>[4x]SPFHLNDAVAIVTGAAAGIGRAIAGTFAKAGASVVVTDLKSEGAEAVAAAIRQAGGKAIGLECNVTDEQHREAVIKAALD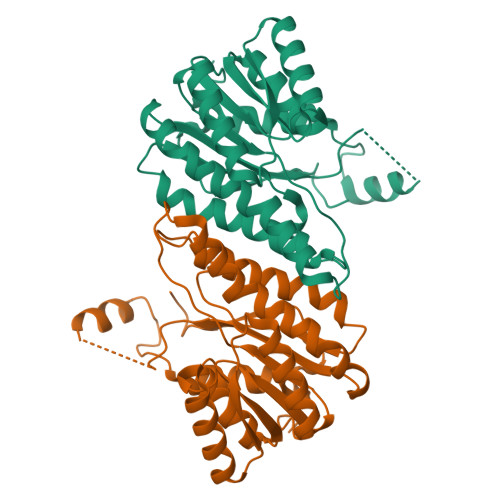QFGKITVLVNNAGGGGPKPFDMPMSDFEWAFKLNLFSLFRLSQLAAPHMQKAGGGAILNISSMAGENTNVRMASYGSSKAAVNHLTRNIAFDVGPMGIRVNAIAPGAIKTDALATVLTPEIERAMLKHTPLGRLGEAQDIANAALFLCSPAAAWISGQVLTVSGGGVQELD2-[(4-azanylcyclohexyl)amino]-7-cyclopentyl-~{N},~{N}-dimethyl-pyrrolo[2,3-d]pyrimidine-6-carboxamide 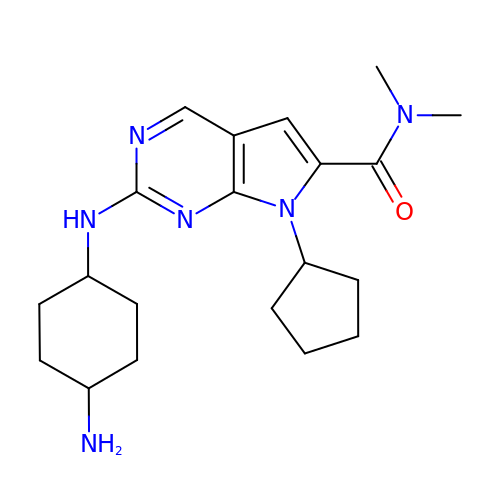| C20 H30 N6 O | HZJPJDOVXYTUTI-SHTZXODSSA-N> MSLTARSVVLSVLLG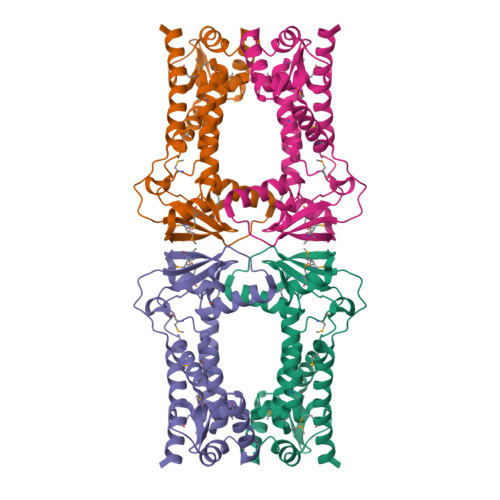AHPAWATASELIQLTADFGIKETTLRVALTRMVGAGDLVRSADGYRLSDRLLARQRRQDEAMRPRTRAWHGNWHMLIVTSIGTDARTRAALRTCMHHKRFGELREGVWMRPDNLDLDLESDVAARVRMLTARDEAPADLAGQLWDLSGWTEAGHRLLGDMAAATDMPGRFVVAAAMVRHLLTDPMLPAELLPADWPGAGLRAAYHDFATAMAKRRDATQLLEVTEGHHHHHH>[7x]AEPVYPDQLRLFSLGQGVCGDKYRPVNREEAQSVKSNIVGMMGQWQISGLANGWVIMGPGYNGEIKPGTASNTWCYPTNPVTGEIPTLSALDIPDGDEVDVQWRLVHDSANFIKPTSYLAHYLGYAWVGGNHSQYVGEDMDVTRDGDGWVIRGNNDGGCDGYRCGDKTAIKVSNFAYNLDP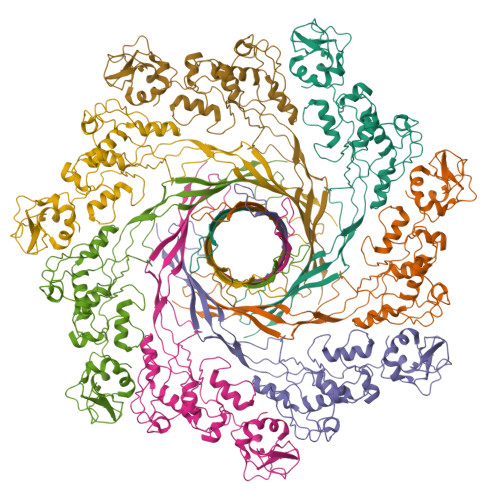DSFKHGDVTQSDRQLVKTVVGWAVNDSDTPQSGYDVTLRYDTATNWSKTNTYGLSEKVTTKNKFKWPLVGETELSIEIAANQSWASQNGGSTTTSLSQSVRPTVPARSKIPVKIELYKADISYPYEFKADVSYDLTLSGFLRWGGNAWYTHPDNRPNWNHTFVIGPYKDKASSIRYQWDKRYIPGEVKWWDWNWTIQQNGLSTMQNNLARVLRPVRAGITGDFSAESQFAGNIEIGAPVPLAA> MLKSSIVLLRRGKPRPRAGMFPEKYRRVPTLLKPQQGGQQYFNEFLIRSANDALEAQQQGYGSAFRVG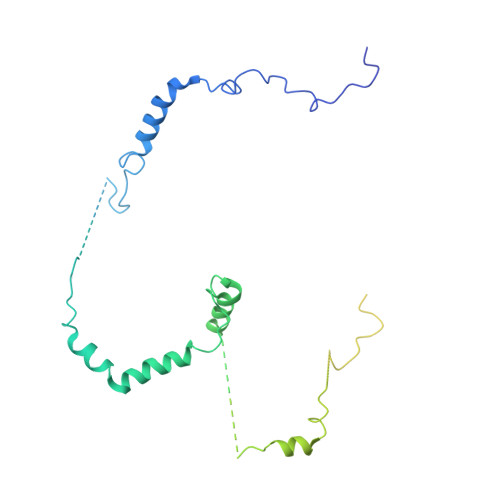GSGAARILADGNATAADGIHDGEISSVHPRLPQADIDGVLQRSRAETIQAELKQLVAQDGFISQRGFNERLWYEQEHHRLRTHGDGVEASPSEVAATAAASSSTAEAVSATGEGRAVPERILGDDYFQSKFGYSLLKGRSPDASAVADNVKAYAQLDLWGEMPMYSRDFVFLYLVSRRRNTYAVAYDYDGKRLLPTYTAGNRGLKGGDRGFRGDGSTDNGHQVTSMYLNDLLPKIREARAASGRPLGRGEKIDLVVRVMGFYNGRQGAVRAVQDRSADFRVRYLEDVTPFPLNGPKMPRGVFR> MSGGDGRGHNTGAHSTSGNINGGPTGLGVGGGASDGSGWSSENNPWGGGSGSGIHWGGGS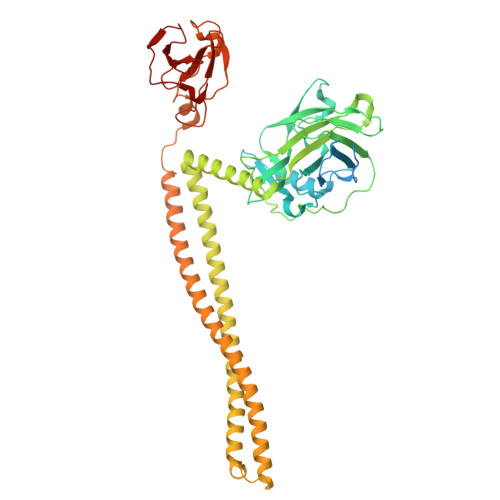GHGNGGGNGNSGGGSGTGGNLSAVAAPVAFGFPALSTPGAGGLAVSISAGALSAAIADIMAALKGPFKFGLWGVALYGVLPSQIAKDDPNMMSKIVTSLPADDITESPVSSLPLDKATVNVNVRVVDDVKDERQNISVVSGVPMSCPVVDAKPTERPGVFTASIPGAPVLNISVNNSTPAVQTLSPGVTNNTDKDVRPAGFTQGGNTRDAVIRFPKDSGHNAVYVSVSDVLSPDQVKQRQDEENRRQQEWDATHPVEAAERNYERARAELNQANEDVARNQERQAKAVQVYNSRKSELDAANKTLADAIAEIKQFNRFAHDPMAGGHRMWQMAGLKAQRAQTDVNNKQAAFDAAAKEKSDADAALSSAMESRKKKEDKKRSAENNLNDEKNKPRKGFKDYGHDYHPAPKTENIKGLGDLKPGIPKTPKQNGGGKRKRWTGDKGRKIYEWDSQHGELEGYRASDGQHLGSFDPKTGNQLKGPDPKRNIKKYL>[3x]MAMSSSAEEVRLDKWL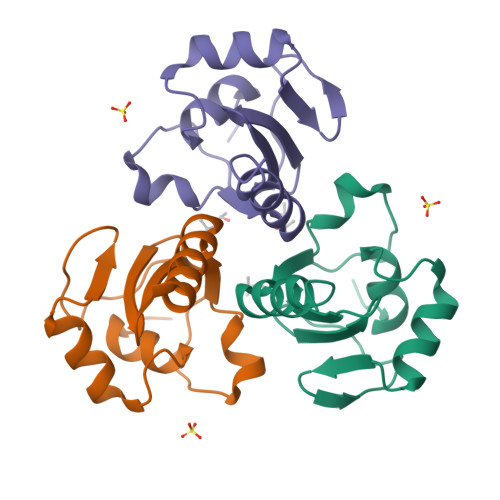WAARFYKTRSLARNMVEGGKVHYNGQRAKPSKSVEIGAQITLRQGHDEKTIIIEKISDQRRGAPEAQQLYRETAKSITKRERNAMMRQLNPSPDRRPDKKQRRDLLKFIHQ>[2x]MDRPAVSGPMDLPIMHDSDRYELVKDIGSGNFGVARLMRDKQSNELVAVKYIERGEKIDENVKREIINHRSLRHPNIVRFKEVILTPTHLAIVMEYASGGELFERICNAGRFSE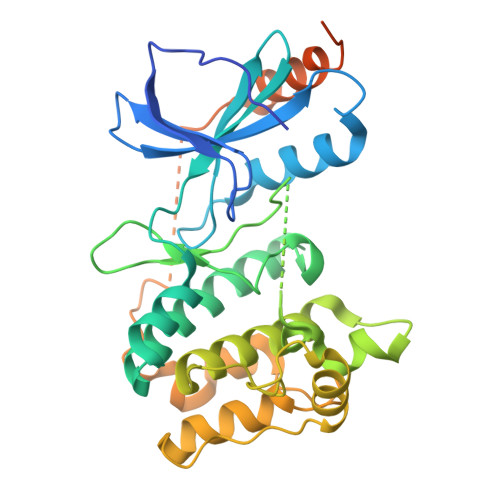DEARFFFQQLISGVSYCHAMQVCHRDLKLENTLLDGSPAPRLKICAFGYSKSSVLHSQPKSTVGTPAYIAPEVLLKKEYDGKVADVWSCGVTLYVMLVGAYPFEDPEEPKNFRKTIHRILNVQYAIPDYVHISPECRHLISRIFVADPAKRISIPEIRNHEWFLKNLPADLMNDNTMTTQFDESDQPGQSIEEIMQIIAEATVPPAGTQNLNHYLTGSLDIDDDMEEDLESDLDDLDIDSSGEIVYAM> MAHH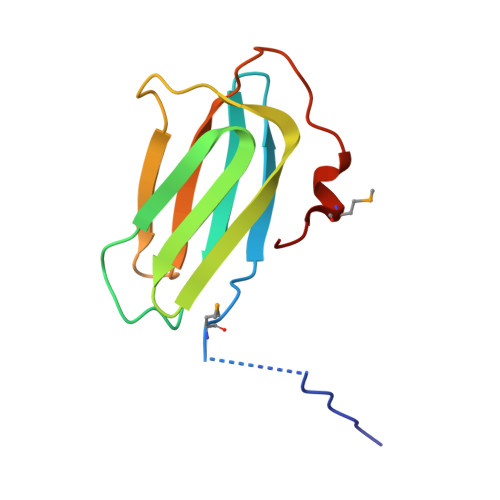HHHHVDDDDKMLTPAFDLSQDPDFLTIAIRVPYARVSEFDVYFEGSDFKFYAKPYFLRLTLPGRIVENGSEQGSYDADKGIFTIRLPKETPGQHFEGLNMLTALLA> AD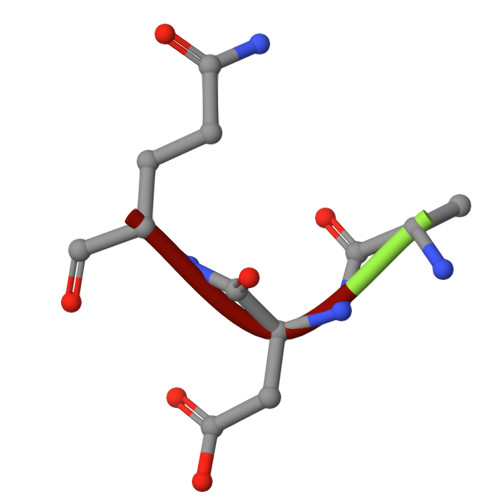Q HOMOBIOTIN | C11 H18 N2 O3 S | 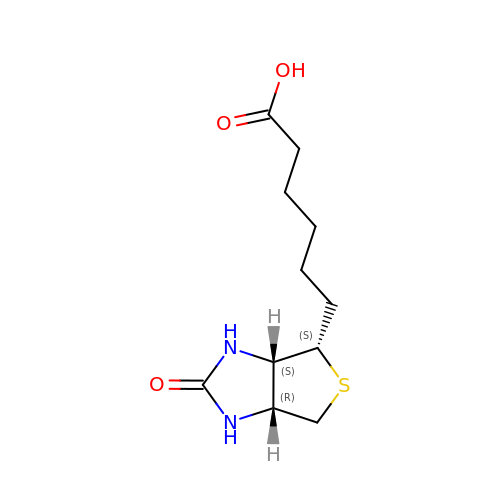CUIOUBJXOZHWNJ-NRPADANISA-N>[4x]ASALWAARRGFVGGNWKCNGTTAKTQELVDMLNSAPVSFEQVDVVVAPPSLFISQVQDSLRQPRVQVAAQDSSTQQAYG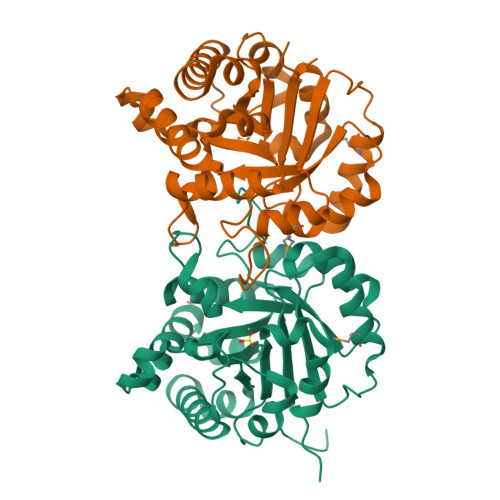AFTGELSPKMIKEKNIPWVVLGHSERRAGFGGQPGESNQVVAKKVRAALNEGLSVILCIGETLEERESGQTQKVLSEQLEAVRQAVPEADAWKSIVIAYEPVWAIGTGKTATAALAQETHRDIRNWLAQAVSPKVAEATRVIYGGSVKGSNAKELFEGEDVDGFLVGGASLTGDFVSIIDAAKQQA> MKIISISETPNHNTMKITLSE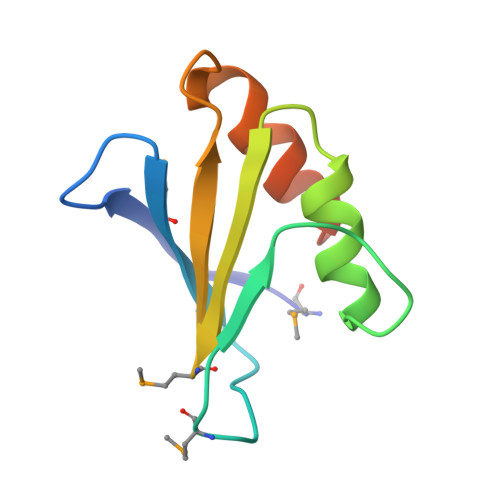SREGMTSDTYTKVDDSQPAFINDILKVEGVKSIFHVMDFISVDKENDANWETVLPKVEAVFELEHHHHHH> MEHHHHHHMPVFHTRT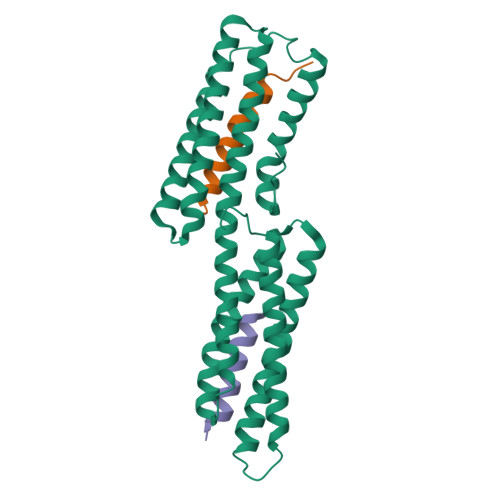IESILEPVAQQISHLVIMHEEGEVDGKAIPDLTAPVAAVQAAVSNLVRVGKETVQTTEDQILKRDMPPAFIKVENACTKLVQAAQMLQSDPYSVPARDYLIDGSRGILSGTSDLLLTFDEAEVRKIIRVCKGILEYLTVAEVVETMEDLVTYTKNLGPGMTKMAKMIDERQQELTHQEHRVMLVNSMNTVKELLPVLISAMKIFVTTKNSKNQGIEEALKNRNFTVEKMSAEINEIIRVLQLTSWDEDAW;>[2x]NHAIYEKAKEVSSALSKVLSKIDDT>[4x]HHHHHHSSGLVPRGSHMRVVVLNWDLLEQVLELGIQPVGAPELSSYVQWVVQPEVPSSVQDIGTRTEPNLEKIAALKPDVILAAGPQQDLLATLGRIAPVVYLPNFSEQDNAAQVAISHFKTLATLFGKEAVAQQKLEAMYARFSELKASLQHAFGDTLPAVVTLRFANPTSVFLYTENSTPQYVLEQLGLSSALPQPP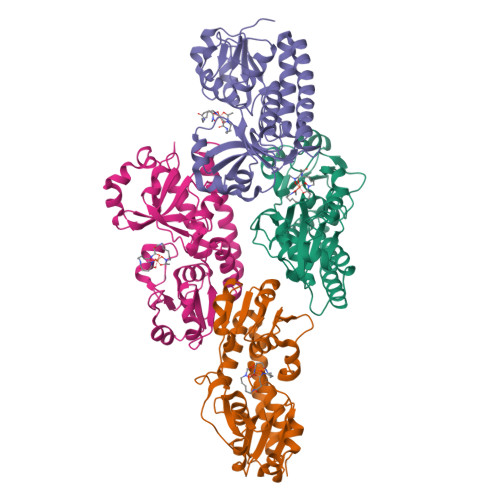KEWGIVQKRLSELQHVEQGYVLYFLPFAEEKKVQKSVLWRAMPFVQAGRVNSVRPVWSYGGAMSLRYSAEAITESLLAVAPQS>TSSKFNECQLNNLNALEPDHRVESEGGLIETWNSQHPELQCAGVTVSKRTLNRNGLHLPSYSPYPQMIIVVQGKGAIGFAFPGCPETFEKPQQQSSRRGSRSQQQLQDSHQKIRHFNEGDVLVIPPGVPYWTYNTGDEPVVAISLLDTSNFNNQLDQNPRVFYLAGNPDIEHPETMQQQQQQKSHGGRKQGQHQQQEEEGGSVLSGFSKHFLAQSFNTNEDTAEKLRSPDDERKQIVTVEGGLSVISPKWQEQEDEDED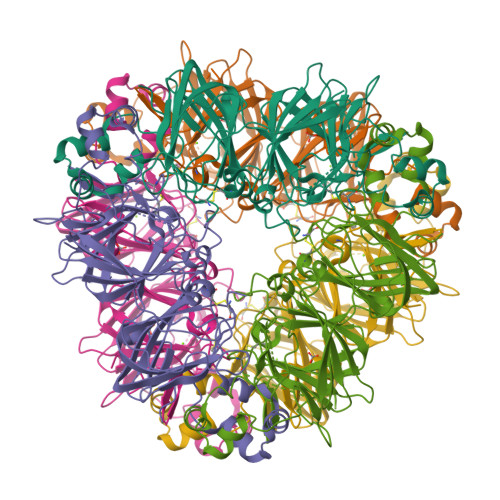EDEEYEQTPSYPPRRPSHGKHEDDEDEDEEEDQPRPDHPPQRPSRPEQQEPRGRGCQTRNGVEENICTMKLHENIARPSRADFYNPKAGRISTLNSLTLPALRQFGLSAQYVVLYRNGIYSPHWNLNANSVIYVTRGKGRVRVVNCQGNAVFDGELRRGQLLVVPQNFVVAEQGGEQGLEYVVFKTHHNAVSSYIKDVFRAIPSEVLSNSYNLGQSQVRQLKYQGNSGPLVNP[2x]>SMTWLPLNPIPLKDRVSMIFLQYGQIDVIDGAFVLIDKTGIRTHIPVGSVACIMLEPGTRVSHAAVRLAAQVGTLLVWVGEAGVRVYASGQPGGARSDKLLYQAKLALDEDLRLKVVRKMFELRFGEPAPARRSVEQLRGIEGSRVRATYALLAKQYGVTWNGRRYDPKDWEKGDTINQCISAATSCLYGVTEAAILAAGYAPAIGFVHTGKPLSFVYDIADIIKFDTVVPKAFEIARRNPGEPDREVRLACRDIFRSSKTLAKLIPLIEDVLAAGEIQPPAPPEDAQPVAIPLPVSLGDAGHRSS[4x];>MMSMLVVVTENVPPRLRGRLAIWLLEVRAGVYVGDVSAKIREMIWEQIAGLAEEGNVV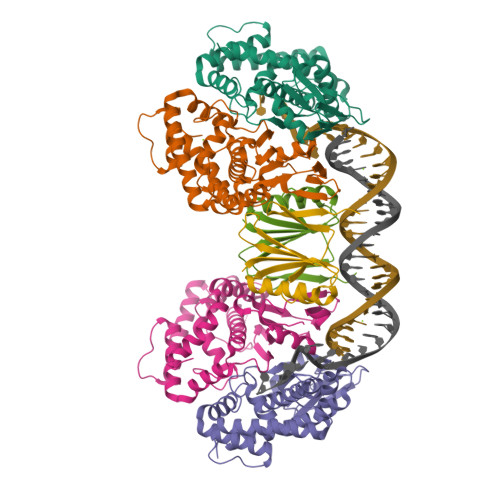MAWATNTETGFEFQTFGLNRRTPVDLDGLRLVSFLPVGSSENLYFQ[2x]>[3x]RLPRETDEEPEEPGRRGS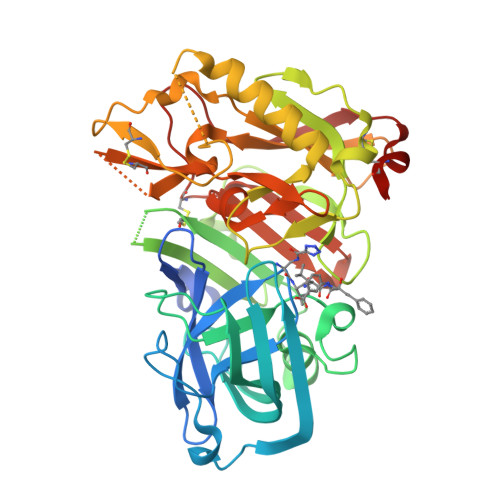FVEMVDNLRGKSGQGYYVEMTVGSPPQTLNILVDTGSSNFAVGAAPHPFLHRYYQRQLSSTYRDLRKGVYVPYTQGKWEGELGTDLVSIPHGPNVTVRANIAAITESDKFFINGSNWEGILGLAYAEIARPDDSLEPFFDSLVKQTHVPNLFSLQLCGAGFPLNQSEVLASVGGSMIIGGIDHSLYTGSLWYTPIRREWYYEVIIVRVEINGQDLKMDCKEYNYDKSIVDSGTTNLRLPKKVFEAAVKSIKAASSTEKFPDGFWLGEQLVCWQAGTTPWNIFPVISLYLMGEVTNQSFRITILPQQYLRPVEDVATSQDDCYKFAISQSSTGTVMGAVIMEGFYVVFDRARKRIGFAVSACHVHDEFRTAAVEGPFVTLDMEDCGYN>ATKLTEEKYELKEGQTLDVKCDYTLEKFASSQKAWQIIRDGEMPKTLACTERPSKNSHPVQVGRIILEDYHDHGLLRVRMVNLQV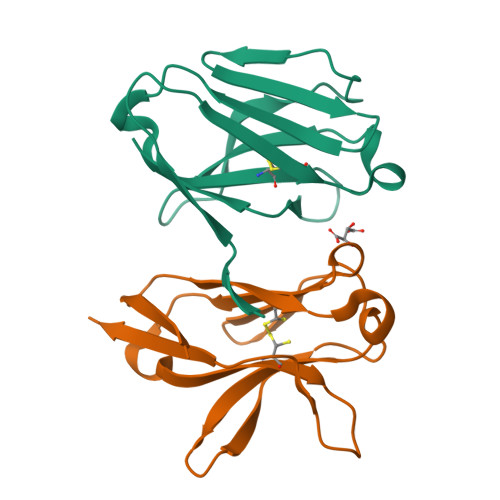EDSGLYQCVIYQPPKEPHMLFDRIRLVVTKGFSG[2x]>STSGRVAVEEVDEEGKFVRLRNKSNEDQSMGNWQIKRQNGDDPLLTYWFPPKFTLKAGQVVTIWAAGAGATHSPPTDLVWKAQNTWGCGNSLRTALINSTGEEVAMRK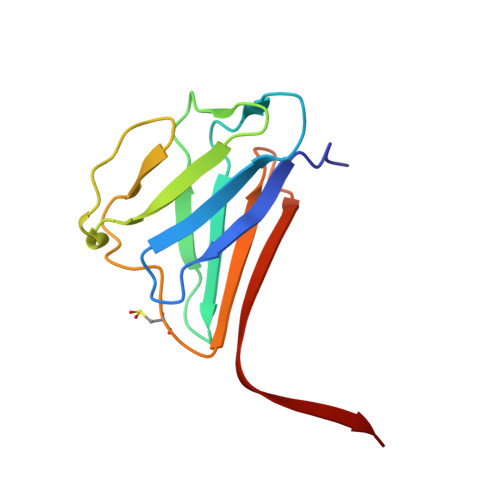LVRSVTVVED[4x]> TKQTVETLM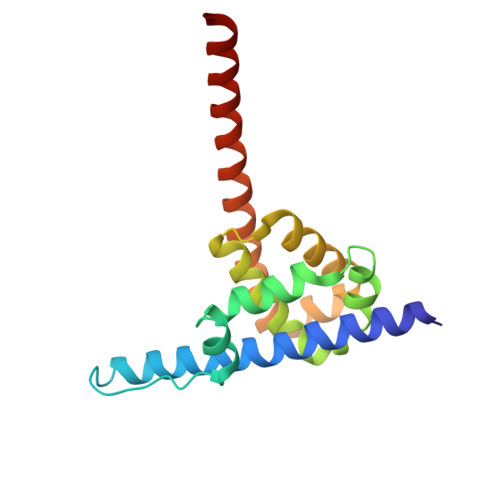AGERIAEALELGMTDLNTIREWEEARQINPNIAPPQRNPIFVALGNIPAETYVLNTLQKIKPASLHDALLVLPFSTIPSLLTFLNLFAQRELNVPLTCRILFFVLKTHHKQIVASRTMRATLEKVRANLRAALRRQKDEMGFNIAALKVVSMQL6-[5-[(2~{S},3~{R},4~{R},5~{S},6~{R})-6-(hydroxymethyl)-3,4,5-tris(oxidanyl)oxan-2-yl]-1~{H}-1,2,4-triazol-3-yl]naphthalene-2-carboxylic 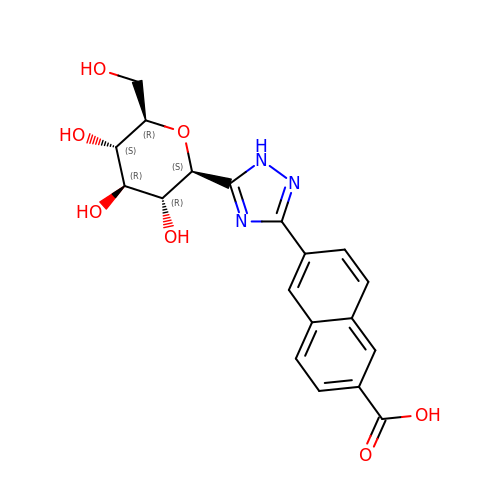acid | C19 H19 N3 O7 | NMFYLVHJQQLQJL-IBEHDNSVSA-N> APPCKGSYFGTENLKSLVLHFLQQYYAIYDSGDRQGLLDAYHDGACCSLSIPFIPQNPARSSLAEYFKDSRNVKKLKDPTLRFRLLKHTRLNVVAFLNELPKTQHDVNSFVVDISAQTSTLLCFSVNGVFKEVDGKSRDSLRAFTRTFIAVPASNSGLCIVNDELFVRNASSEEIQRAFAMPAPTPSSSPVPTLSPEQQEMLQA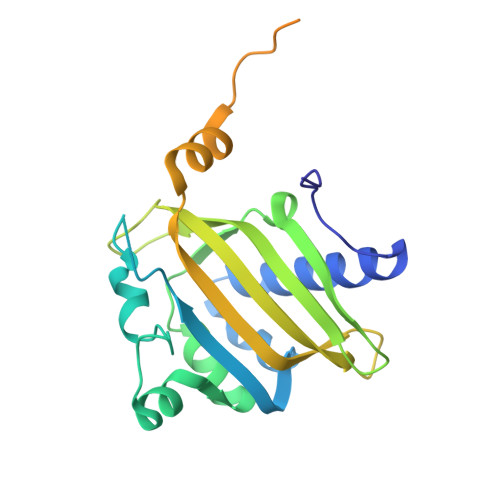FSTQSGMNLEWSQKCLQDNNWDYTRSAQAFTHLKAKGEIPEVAFMK>MSGAPPPSSGFAPRSYGQQPLSHAPRSSMMSVEYDGIPLPPPSIRSCGSQQYVTSYIPTGAAFPPSSVQDMISSMKSYASATDLVRTYSEIPSVEEALSTLDRAAAALNARRYRDALKLYLEGGYAMANVAERQANPKICNLLTSKGFETLNWCARLCDWIEGRIKEKHPRPGVHKVGIPVSNWDEDWVGPFMDEEEARRMWYTPVYCPHPIDFSNLGYRLRCVETGRRPRLMICITMYNEGPQQLKATLKKLANNLAYLKEQMPGDEKSLTGAFAGDDVWQNVLVCIVADGREQVHPKTLDYLEAIGLYDEDLLTINSAGIGAQCHLFEHTLQLSVNGKCLLPIQTVFALKENKASKLDSHHWYFNAFAEQIQPEYTAVMDVGTMLTKSALYHLLFAFERNHQIGGACGQLTVDNPFENLSNWVISAQHFEYKISNILDKSLESCFGFISVLPGAFSAYRYEAIRGAPLDAYFQTLNIELDVLGPFIGNMYLAEDRILSFEVVARKNCNWTMHYVKDAVARTDVPHDLVGLISQRKRWLNGAFFATLFSIWNWGRIYSESKHTFVRKMAFLVFYVYHLLYTAFGFFLPANLYLALFFIVFQGFQQNRLEFIDTSEYSQTVLDCAVYIYNFSYLFGLLMLIIIGLGNNPKHMKLTYYFVGAVFGLMMMLSSLVGAGIFFSTPATVHSIVVSILTVGVYFIASALHGEVHHIFMTFTHYTALIPSFVNIFTIYSFCNLQDLSWGTKGLHDDPLLAASLDETEKGDFKDVIAKRRALEELRREEKERVENRKKNFEAFRTNVLLTWAFSNLIFALFVVYFASSSTYMPVLYIFVASLNTCRLLGSIGHWVYIHTEGLRGRVIDKSECGNGTGRYPQNSYVQLEEHYAALAEDQRTYASGRTNASVRTVNDVSSAALVPRGSHHHHHH[2x]

Chitin is synthesized by chitin synthase (CHS), a membrane-integrated protein belonging to the glycosyltransferase family 2, consisting of a glycosyltransferase (GT) domain and a transmembrane (TM) region. CHS incorporates UDP-N-acetylglucosamine (UDP-GlcNAc) onto the acceptor molecule to form the nascent chitin, which has been validated by in vitro activity assays. In this study, we demonstrated that Phytophthora sojae chitin synthase (PsCHS) exhibits processivity and functions as a bifunctional enzyme, capable of catalyzing both the synthesis and membrane translocation of chitin. A short N-terminal domain (NTD) exists in some CHSs, like Phytophthora sojae chitin synthase 1 (PsCHS1), to stabilize the dimerization.

To capture the structure of chitin-bound PsCHS, we incubated the enzyme in the presence of UDP-GlcNAc and Mn2+ for 15 min or 40 min before cryo-EM sample preparation. However, only a UDP- and Mn2+-occupied structure was resolved for both samples with overall resolutions of 3.20 Å and 2.94 Å, respectively. Unfortunately, only the PsCHS structure with the UDP/Mn2+ bound was obtained, which represents the competitive substrate binding or post-translocation state. PsCHS forms a dimer, as previously reported. Each protomer contains a long transmembrane helix, with its N-terminal region extending to the adjacent protomer, stabilizing the dimer with the interaction interface located at the GT domain as well as the TM region. UDP and Mn2+ are positioned in the reaction cavity of the GT domain, where PsCHS stabilizes UDP via hydrogen bonding and π-π stacking interactions. Q535 of the amphipathic interface helices (IF2) forms two hydrogen bonds with the pyrophosphate group, while other hydrogen bonds occur between the uridine portion of UDP and the GT domain. Specifically, E241, D382, V383, T237, and Y239 form hydrogen bonds with the ribose moiety, while D291, K355, K358, and S361 bond with the uracil moiety. Y239 also participates in π-π stacking with the uracil ring and Mn2⁺ coordinates with the pyrophosphate group. IF1 and IF2 connect the GT domain and transmembrane helices, framing the entrance of the potential chitin translocation channel.> GIEDLITEVAQGALTLSLPKQQDSLPDTKASGPAHSKEVPALTAVETGATNPLVPSDTVQTRHVIQRRSRSESTIESFFARGACVAIIEVDNEEPTTRA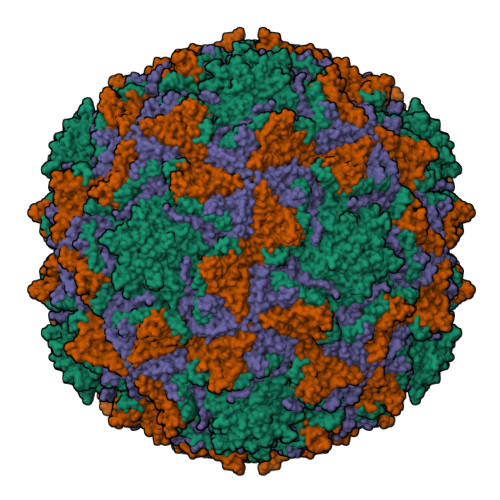QKLFAMWRITYKDTVQLRRKLEFFTYSRFDMELTFVVTANFTNTNNGHALNQVYQIMYIPPGAPTPKSWDDYTWQTSSNPSIFYTYGAAPARISVPYVGLANAYSHFYDGFAKVPLKTDANDQIGDSLYSAMTVDDFGVLAIRVVNDHNPTKVTSKVRIYMKPKHVRVWCPRPPRAVPYYGPGVDYKDNLNPLSEKGLTTY;> MGAQVSSQKVGAHENSNRAYGGSTINYTTINYYKDSASNAASKQDYSQDPSKFTEPLKDVLIKTAPALNSPNVEACGYSDRVLQLTIGNSTITTQEAANSVVAYGRWPEFIRDDEANPVDQPTEPDVATCRFYTLDTVMWGKESKGWWWKLPDALRDMGLFGQNMYYHYLGRSGYTVHVQCNASKFHQGALGVFAIPEYCLAGDSDKQRYTSYANANPGEKGGKFYSQFNRDTAVTSPKREFCPVDYLLGCGVLLGNAFVYPHQIINLRTNNSATIVLPYVNAMAIDSMVKHNNWGIAILPLSPLDFAQESSVEIPITVTIAPMCSEFNGLRNVTAPKFQ;> GLPVLNTPGSNQYLTSDNYQSPCAIPEFDVTPPIDIPGEVKNMMELAEIDTMIPLNLENTKRNTMDMYRVTLSDSADLSQPILCFSLSPASDPRLSHTMLGEVLNYYTHWAGSLKFTFLFCGSMMATGKILVAYAPPGAQPPTSRKEAMLGTHVIWDLGLQSSCTMVVPWISNVTYRQTTQDSFTEGGYISMFYQTRIVVPLSTPKSMSMLGFVSACNDFSVRLLRDTTHISQSALPQ> GDEPPQSPWDRVKDLATVYVDVLKDSGRDYVSQFEGSALGKQLNLKLLDNWDSVTSTFSKLREQLGPVTQEFWDNLEKETEGLR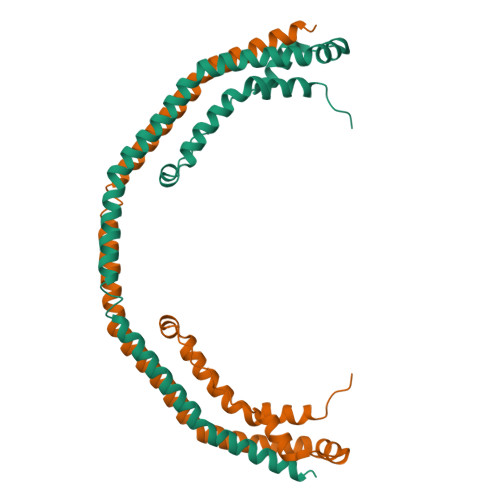QEMSKDLEEVKAKVQPYLDDFQKKWQEEMELYRQKVEPLRAELQEGARQKLHELQEKLSPLGEEMRDRARAHVDALRTHLAPYSDELRQRLAARLEALKEN>DAAQPALLQYHYDCGDFGMQLLAYPTRGRTVHFKVLDEFGTRFEVANCSICMHWLNTGEDGGLIFSAGYEGCHVLVKDGRYVLRVQLEEMLLSGVVAASYEVQMTCPRPAGYEILRDEKVHHHHHHHHQRPDRGNS[2x]

Vertebrate oocytes are surrounded by a specialised extracellular coat that is referred to as zona pellucida in mammals (ZP) and vitelline envelope in non-mammals (VE). Although their fine morphological appearance differs between classes, all vertebrate egg coats consist of filaments made up of a variable number of glycoprotein components that polymerise using a common ZP module. Accordingly, a recombinant construct corresponding to the predicted ZP-N1 domain of cZP1 (cZP1-N1) is secreted both as a monomeric and a disulphide-bonded dimer, whereas a protein encompassing the trefoil domain and C-terminal ZP module of cZP1 (cZP1L600-R958) does not form intermolecular disulphides. Thus, by recapitulating the oligomeric status of full-length cZP1, cZP1-N1 harbours its cross-linking function.

Accordingly, whereas mutation of cZP1-N1 N65 or hZP1-N1 N76 drastically reduces protein secretion, a cZP1 N121Q mutant is secreted as well as the wild-type and—because of its higher homogeneity—was used for crystallisation trials in parallel with hZP1-N1. Whereas the latter did not crystallise, we could grow crystals of cZP1-N1 expressed in human embryonic kidney (HEK) 293S GnTI- cells and treated with Endoglycosidase (Endo) H, as well as the same protein expressed in HEK293T cells. Remarkably, although they all contain the same C66-C66 cross-link, the moieties of the cZP1-N1 homodimers observed in our crystal forms adopt three distinct relative orientations. These correspond to an asymmetric interface in the case of deglycosylated cZP1-N1 (whose crystallographic asymmetric unit contains a homodimer) and two related but not identical interfaces in the crystal of glycosylated cZP1-N1 (whose asymmetric unit also contains two copies of the protein (chains A and B) that, however, make intermolecular cross-links with symmetry-related copies of themselves (A′ and B′)). All the cZP1 cross-links have small interface areas that range from 330/412 Å2 (A-A′/B-B′ dimers of glycosylated cZP1-N1) to 575 Å2 (deglycosylated cZP1-N1 dimer). Distinct sets of interactions mediated by these residues underlie the different homodimer interfaces: for example, in the deglycosylated cZP1-N1 homodimer, C′ strand F61(A) interacts aromatically with W72(B) and I68(A) packs against I68(B); on the other hand, in both glycosylated cZP1-N1 homodimers, the latter interaction is missing because I68 interacts hydrophobically with F61 of the opposite subunit. Additional contacts between residues in the ab loop/β-strand B region and amino acids in the cd loop stabilises the asymmetric structure of the deglycosylated cZP1-N1 cross-link; in particular, invariant Q38(B) stacks against highly conserved F57(A) and also makes water-mediated hydrogen bonds with the side chains of T59(A) and invariant D55(A).>[2x]MEGMLKGEGPGPLPPLLQQYVELRDQYPDYLLLFQVGDFYECFGEDAERLARALGLVLTHKTSKDFTTPMAGIPLRAFEAYAERLLKMGFRLAVADQVEPAEEAEGLVRREVTQLLTPGTLLQESLLPREANYLAAIATGDGWGLAFLDVSTGEFKGTVLKSKSALYDELFRHRPAEVLLAPELLENGAFLDEFRKRFPVMLSEAPFEPEGEG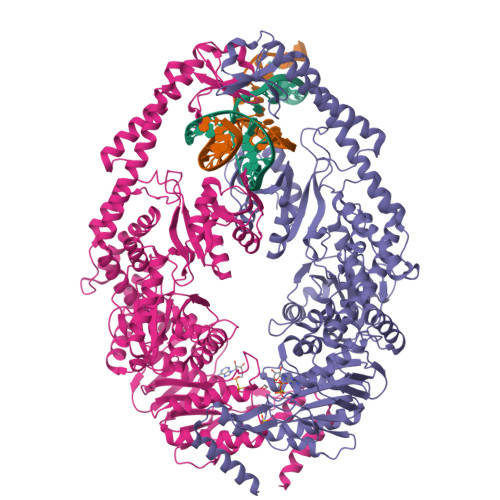PLALRRARGALLAYAQRTQGGALSLQPFRFYDPGAFMRLPEATLRALEVFEPLRGQDTLFSVLDETRTAPGRRLLQSWLRHPLLDRGPLEARLDRVEGFVREGALREGVRRLLYRLADLERLATRLELGRASPKDLGALRRSLQILPELRALLGEEVGLPDLSPLKEELEAALVEDPPLKVSEGGLIREGYDPDLDALRAAHREGVAYFLELEERERERTGIPTLKVGYNAVFGYYLEVTRPYYERVPKEYRPVQTLKDRQRYTLPEMKEKEREVYRLEALIRRREEEVFLEVRERAKRQAEALREAARILAELDVYAALAEVAVRYGYVRPRFGDRLQIRAGRHPVVERRTEFVPNDLEMAHELVLITGPNMAGKSTFLRQTALIALLAQVGSFVPAEEAHLPLFDGIYTRIGASDDLAGGKSTFMVEMEEVALILKEATENSLVLLDEVGRGTSSLDGVAIATAVAEALHERRAYTLFATHYFELTALGLPRLKNLHVAAREEAGGLVFYHQVLPGPASKSYGVEVAAMAGLPKEVVARARALLQAMAAR> XPLDLCYWASLHCIV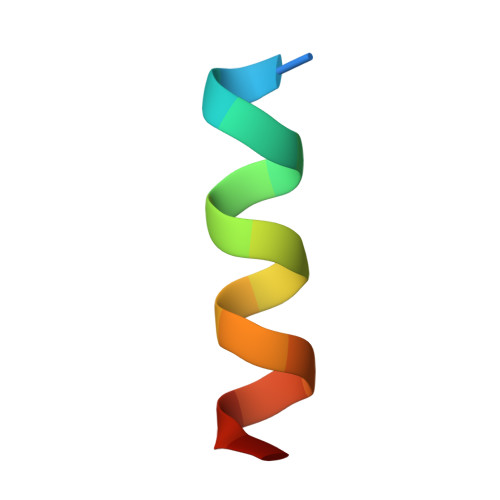SX>AKVAVLGASGGIGQPLSLLLKNSPLVSRLTLYDIAHTPGVAADLSHIETRATVKGYLGPEQLPDCLKGCDVVVIPAGVPRKPGMTRDDLFNTNATIV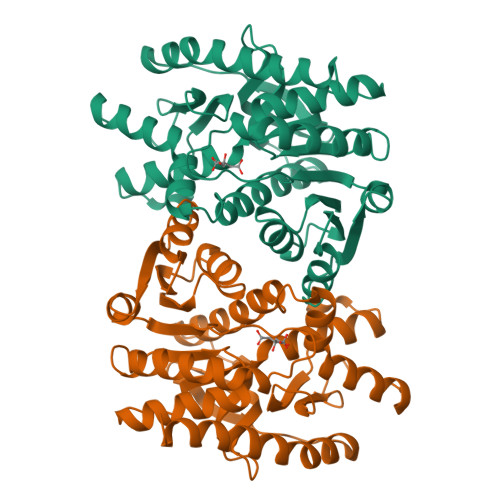ATLTAACAQHCPDAMICIISNPVNSTIPITAEVFKKHGVYNPNKIFGVTTLDIVRANAFVAELKGLDPARVSVPVIGGHAGKTIIPLISQCTPKVDFPQDQLSTLTGRIQEAGTEVVKAKAGAGSATLSMAYAGARFVFSLVDAMNGKEGVVECSFVKSQETDCPYFSTPLLLGKKGIEKNLGIGKISPFEEKMIAEAIPELKASIKKGEEFVKNMK[4x]>[3x]NPCLTGPRTCK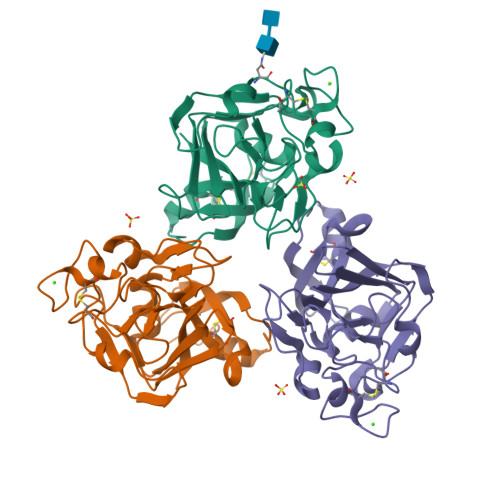DLLDRGHFLSGWHTIYLPDCRPLTVLCDMDTDGGGWTVFQRRVDGSVDFYRDWATYKQGFGSRLGEFWLGNDNIHALTAQGTSELRVDLVDFEDNYQFAKYRSFKVADEAEKYNLVLGAFVEGSAGDSLTFHNNQSFSTKDQDNDLNTGNCAVMFQGAWWYKNCHVSNLNGRYLRGTHGSFANGINWKSGKGYNYSYKVSEMKVRPA> MVTVEATENL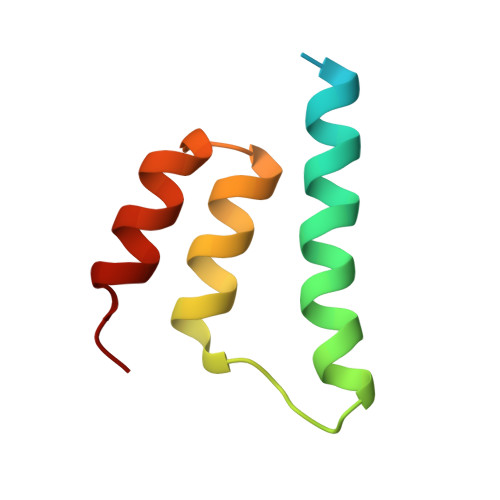LSITLEELKKRREAVDAVISTHALEGIALHPKTLKILEGYARGNTSLEEFNTLMDNAKL>MTWEHNEFMQMTVKPFLIPADKVAHVQPGNYLDHALLVLTKTGYSAIPVLDTSYKLHGLISMTMMMDAILGLERIEFERLETMKVEEVMNRNIPRLRLDDSLMKAVGLIVNHPFVCVENDDGYFAGIFTRREVLKQLNKQLHRPNGGRKL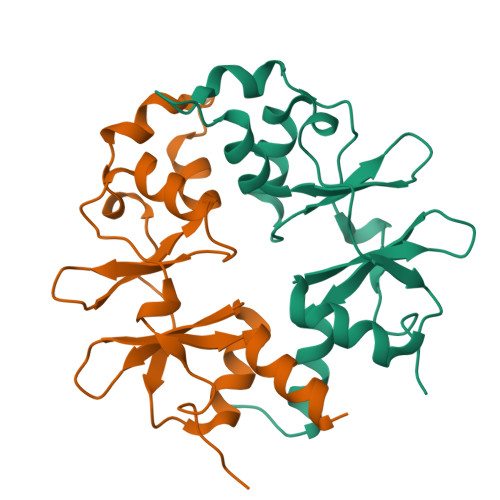GRKEAEQ[2x]>[4x]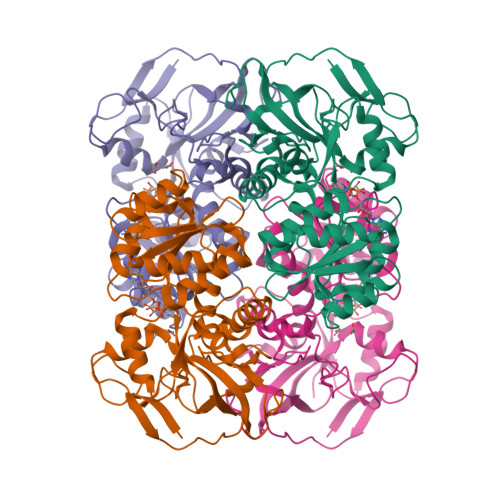MKAVQYTEIGSEPVVVDIPTPTPGPGEILLKVTAAGLCYSDIHVMDMPAAQYAFGLPLTLGHEGVGTVAELGEGVTGFGVGDAVAVYGPWGCGACHACARGRENYCTRAADLGITPPGLGSPGSMAEYMIVDSARHLVPIGDLDPVAAAPLTDAGLTPYHAISRVLPLLGPGSTAVVIGVGGLGHVGIQILRAVSAARVIAVDLDDDRLALAREVGADAAVKSGAGAADAIRELTGGQGATAVFDFVGAQSTIDTAQQVVAVDGHISVVGIHAGAHAKVGFFMIPFGASVVTPFAGTRSELMEVVALARAGRLDIHTETFTLDEGPAAYRRLREGSIRGRGVVVPTSHHHHH> GAGCAGACGTGACTCCACTCA;> A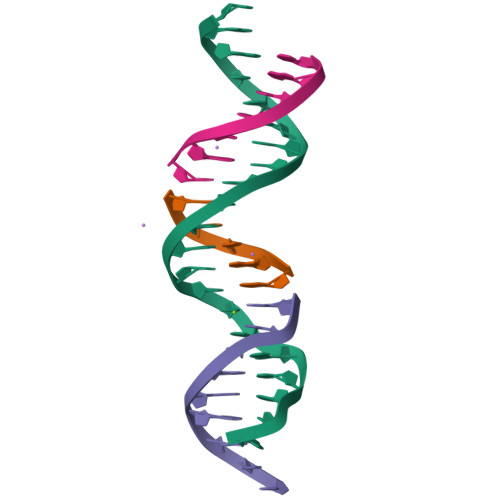GTCA;> TCTGAGTGG;> CGTCTGC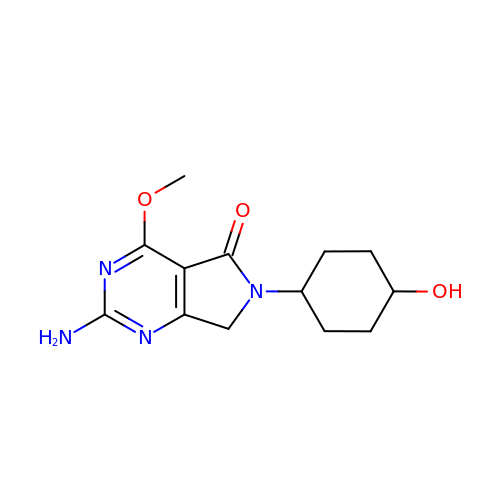2-azanyl-4-methoxy-6-(4-oxidanylcyclohexyl)-7~{H}-pyrrolo[3,4-d]pyrimidin-5-one | C13 H18 N4 O3 | ARZZIEXRMVZGIF-OCAPTIKFSA-N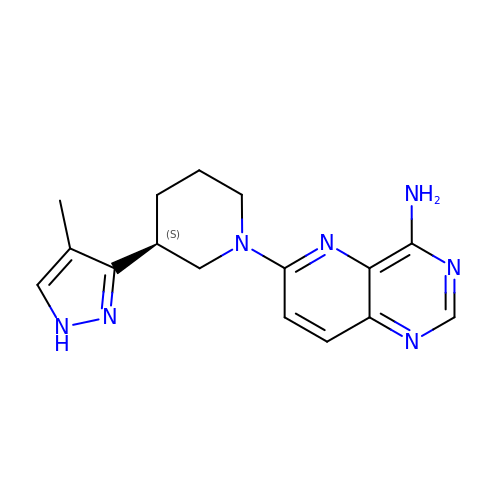6-[(3S)-3-(4-methyl-1H-pyrazol-3-yl)piperidin-1-yl]pyrido[3,2-d]pyrimidin-4-amine | C16 H19 N7 | NUOOXGXOVSCCHC-NSHDSACASA-N> GSMAPRAGFDAEQVRDKARKDLLHLLEGVRGKKNLVIEKDLAGPLGVIVKASTLRDYGVDNFFFLENKNTGTSQRNIVFIARGESVRNAHAIAAQIKRIQRESQTSHDFHIFWVPRRTLFSDKVLEEAGVLGDANISELPLYFFPLERDVLSLELNDSFRDLYLAKDPTPVFLLSRALMGIQKKHGLFPRIIGKGENAKRVADLLSRMRQELLAGEEAGESDRAGLSPSTTIESVIIIDREVDFVTPLLTQLTYEGLIDEYFGIQNNQTDVDAVIVGAPAQSAASTSTAVPT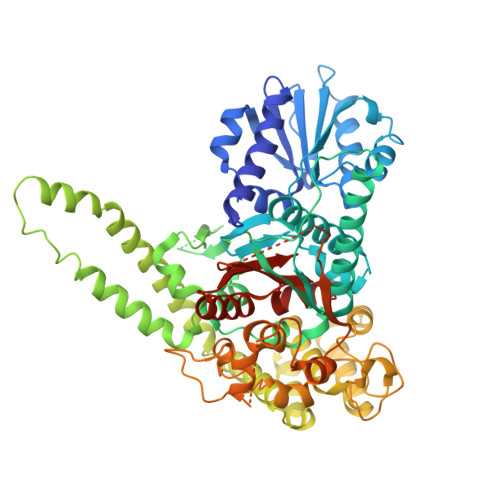NSSQSRKRKIQLDGSDSLYSQLRDANFAIVGSLLNTVARRLKSDYESRHNTKTTAELKEFVKKLPGYQAEQQSLKIHSNIAEEIINYTRTEIFNKLLEVQQNLAAGADPSSQFDSIEELVARDTPLPQVLRLLCLYSCISGGIKTKELDHFRRLVLQGYGHQHLLTLHNLERLQMFLSKSSPLASMITMSGSSGGPDQKTNYTYLRKQLRLIVDEVNEQDPNDIAYVYSGYAPLSIRLVQCVLQKQYLLSITKGSGTVIAAGPVAGGGAQGWKGFEEIVKHARGPTFDEIQKGEDKAVKARALLSGSSGDKKTVFVVFVGGITFTEIAALRFIAKQEEARRNIVICTTSIINGNRMMNAAIETATFEKTTVTTAAAQ> HMSNYTVKIKNSAKSDLKKIKHSY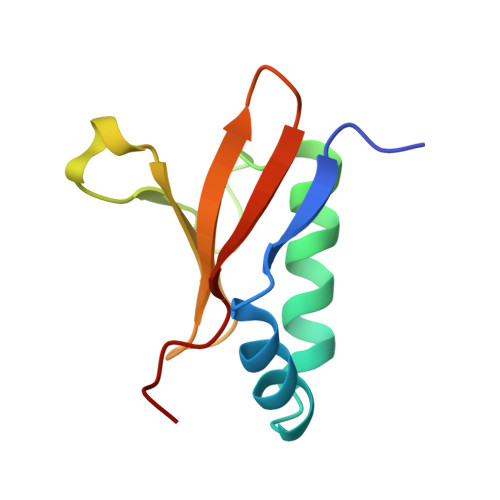LKKSFLEIVETLKNDPYKITQSFEKLEPKYLERYSRRINHQHRVVYTVDDRNKEVLILSAWSHYD>[2x]GSEAAGGEQRELLIQRLRAAVHYTTGCLCQDVAEDKGVLFSKQTVAAISEITFRQCENFARDLEMFARHAKRSTITSEDVKLLARRSNS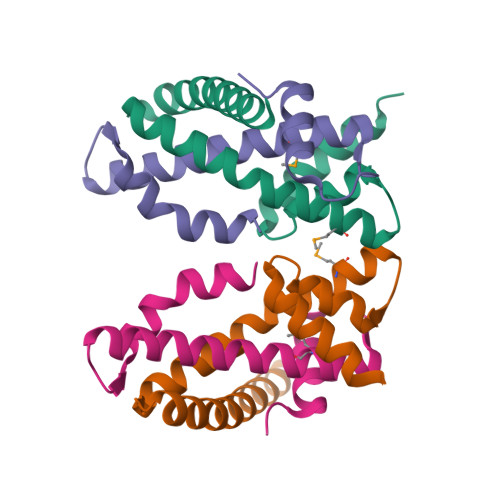LLKYITQKSDELASSNME;>[2x]GYEEREGGFRKETVERLLRLHFRDGRTRVNGDALLLMAELLKVFVREAAARAARQAQAEDLEKVDIEHVEKVLPQLLLDFV The icosahedral capsid contains 60 copies of a protomeric unit composed of four proteins, VP1-4. Enteroviruses are unique in harbouring a lipid molecule (pocket factor) within a pocket in the VP1 β-barrel, which lies below the surface of a deep depression encircling each fivefold axis, termed the canyon. The binding of such receptors can trigger pocket factor release and viral expansion, leading to externalization of the N-terminus of VP1 followed by VP4 to form a pore in the endo/lysosome membrane through which the genome is thought to be subsequently released. Here, we have determined three cryo-EM structures following mixing of CV-A10 Kowalik strain with KRM1: the CV-A10 mature virus, a disassembly intermediate A-particle and the mature virus in complex with KRM1.

The expanded intermediate is termed the A-particle prior to genome release and B-particle subsequent to genome release. Conformational changes relative to the mature capsid are observed in the residues preceding strand B of VP2 which in the A-particle adopt a helical structure, whilst the VP3 GH loop becomes disordered. The previously internal N-terminus of VP1 now traverses the capsid from the region of RNA interaction, via the “off-axis” channel becoming disordered or cleaved beyond the last visible residue, 66. This recapitulates the externalization of VP1 visualized in Poliovirus and CV-A1625,26 rendering the inter-pentamer interface less stable and compromising capsid integrity. The A-particles showed no evidence of bound KRM1. The reduced occupancy of pocket factor in the complexed-virus particles and the presence of both unbound and expanded full particles suggests that receptor binding triggers pocket factor release, initiating the cascade of conformational changes that produces expanded A-particles. These A-particles are unable to bind receptor and are ready to uncoat by releasing the genome.

> GDPVEDIIHDALSSTVRRAITSGQDVNTAAGTAPSSHRLETGRVPALQAAETGATSNATDENMIETRCVMNRNGVLEATISHFFSRSGLVGVVNLTDGGTDTTGYAVWDIDIMGFVQLRRKCEMFTYMRFNAEFTFVTTTENGEARPFMLQYMYVPPGAPKPTGRDAFQWQTATNPSVFVKLTDPPAQVSVPFMSPASAYQWFYDGYPTFGQHPETSNTTYGQCPNNMMGTFAVRVVSRVASQLKLQTRVYMKLKHVRAWIPRPIRSQPYLLKNFPNYDSSKITYSARDRASIKQANM;> SPSVEACGYSDRVAQLTVGNSSITTQEAANIVLAYGEWPEYCPDTDATAVDKPTRPDVSVNRFYTLDSKMWQENSTGWYWKFPDVLNKTGVFGQNAQFHYLYRSGFCLHVQCNASKFHQGALLVAVIPEFVLAGRGSNTKPNEAPHPGFNTTFPGTAGASFNDPYVLDSGVPLSQSLIYPHQWINLRTNNCATIIVPYINAVPFDSAINHSNFGLIVVPVSPLKYSSGATTAIPITVTIAPLNSEFGGLRQAVSQ;> GLPTELRPGTNQFLTTEDDTAAPILPGFSPTPSIHIPGEVRSLLELCRVETILEVNNTTDATGLNRLLIPVSAQNKADELCAAFMVDPGRIGPWQSTLVGQICRYYTQWSGSLKVTFMFTGSFMATGKMLIAYSPPGSAQPANRETAMLGTHVIWDFGLQSSVSLVIPWISNTHFRTAKTGGNYDYYTAGVVTLWYQTNYVVPPETPGEAYIIAMGAAQDNFTLKICKDTDEVTQQAVLQ~{N}-quinolin-6-ylbenzamide | C16 H12 N2 O | 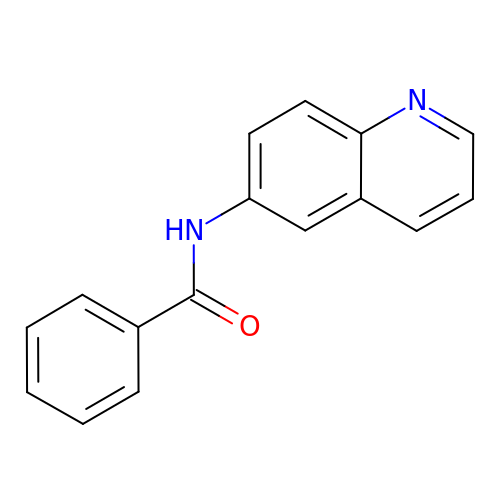WQBDHSKBYRWNNN-UHFFFAOYSA-N>[4x]MGSSPSLEQDDGDEETSVVIVGKISFCPKDVLGHGAEGTIVYRGMFDNRDVAVKRILPECFSFADREVQLLRESDEHPNVIRYFCTEKDRQFQYIAIELCAATLQEYVEQKDFAHLGLEPITLLQQTTSGLAHLHSLNIVHRDLKPHNILISMPNAHGKIKAMISDFGLCKKLAVGRHSFSRRSGVPGTEGWIAPEMLSEDCKENPTYTVDIFSAGCVFYYVISEGSHPFGKS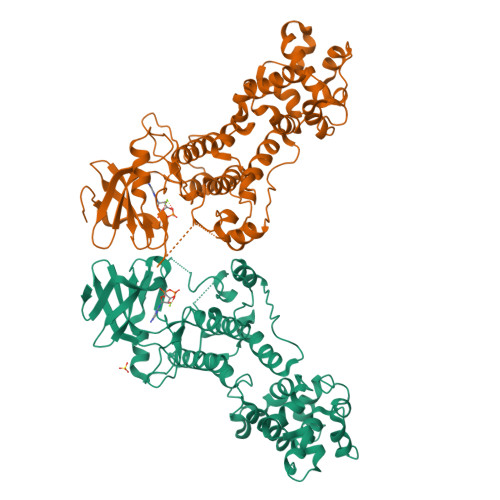LQRQANILLGACSLDCLHPEKHEDVIARELIEKMIAMDPQKRPSAKHVLKHPFFWSLEKQLQFFQDVSDRIEKESLDGPIVKQLERGGRAVVKMDWRENITVPLQTDLRKFRTYKGGSVRDLLRAMRNKKHHYRELPAEVRETLGTLPDDFVCYFTSRFPHLLAHTYRAMELCSHERLFQPYYFHEPPEPQPPVTPDAL>[112x]MGLFDRIKRVVSSNLNDLVNKAEDPEKMLEQAILEMQEDLVQLRQGVAQAIAAQKRSEKQYNDAQNEINKWQRNAQLALQKGDENLARQALERKKTYTDTSAALKASLDTQSTQVETLKRNLIQLESKISEAKTKKEMLKARITTAKAQEQLQGMVRGMNTSSAMSAFERMEEKVLMQESRAQALGELAGADLETQFAQLEGGSDVDDELAALKAQMLPPATPVTQAQLPPQQETTPAKSNEVVDAELDSLRKQLDQL

Proteins that perform these functions include Vipp1/IM30 in photosynthetic plastids, PspA in bacteria, and ESCRT-III in eukaryotes. Here, using a combination of evolutionary and structural analyses, we show that these protein families are homologous and share a common ancient evolutionary origin that likely predates the last universal common ancestor. This homology is evident in cryo-electron microscopy structures of Vipp1 rings from the cyanobacterium Nostoc punctiforme presented over a range of symmetries. Rings have an inner lumen that is able to bind and deform membranes.

Reconstructions were also generated for the other six symmetries and complete ring models built. Rungs are maximally constricted at the top and bottom with internal lumen diameters of 14 nm and 15.7 nm, and widest at the ring equator between rungs 3 and 4 with an internal diameter of 17.5 nm. This unique asymmetric curvature is a feature of all Vipp1C11–C17 ring symmetries. The analysis of different ring symmetries, ranging from C11–C17, provides us with a view of the structural flexibility that enables Vipp1, PspA, and ESCRT-III family members to perform their functions. Furthermore, as each ring comprises between 5–7 rungs stacked together to build a dome-shaped architecture, these asymmetric structures provide us with a glimpse of the structural features that enable filament tilt in the context of an ESCRT-III-like polymer. Consistent with this, Interfaces 1 and 3 linking the top two rungs were poorly resolved in Vipp1C11–C17 rings, indicating a weak interaction once the limiting geometry is reached. When membrane was modeled into the Vipp1C11–C17 structures as a 4-nm bilayer, sequential constriction was observed with the membrane lumen reaching ∼3 nm within Vipp1C11.> GAMDPRVTMNEFEYLKLLGKGTFGKVILVKEKATGRYYAMKILKKEVIVAKDEVAHTLTENRVLQNSRHPFLTALKYSFQTHDRLCFVMEYANGGELFFHLSRERVFSEDRARFYGAEIVSALDYLHSEKNVVYRDL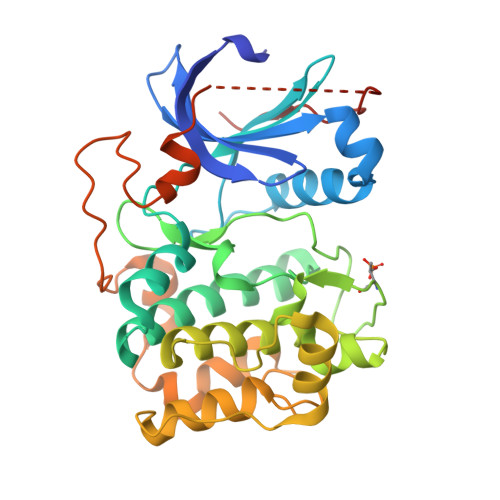KLENLMLDKDGHIKITDFGLCKEGIKDGATMKTFCGTPEYLAPEVLEDNDYGRAVDWWGLGVVMYEMMCGRLPFYNQDHEKLFELILMEEIRFPRTLGPEAKSLLSGLLKKDPKQRLGGGSEDAKEIMQHRFFAGIVWQHVYEKKLSPPFKPQVTSETDTRYFDEEFTAQMITITPPDQDDSMECVDSERRPHFPQFDYSASSTA> MSTIEHQMHLEKLYNKNQLLPRMRQEFEENSGIDFKAFFAHIGIDYKFGIDAMVQMALHKRADLPTLVGTLRHHCKSAQEVADNLFKMASEDCFNFDPTIDKFIVIYTISDDVQHELDSFQYPLPMVVRPKLLTKNYGTGYFTCNKSVILKKNHTDDDICLDHLNRMNKIPLSINWDVAHMVKNEWANLDKPKEGETRQEFEKRVRAFQKYDRTAHEVMGLLTQEGNKFYLTHRPDKRGRTYS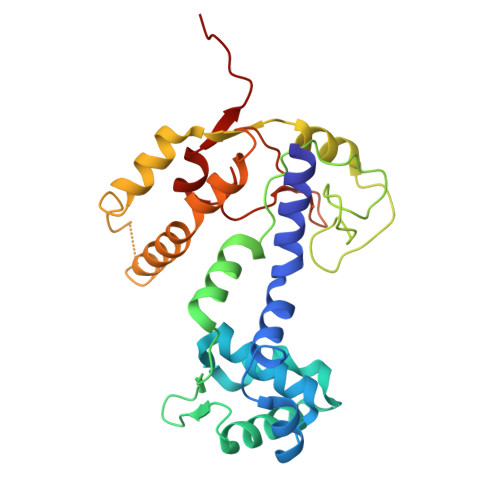QGYHVNYQGTSWNKAVLEFAEKEVID>SNAMFTTVITPRVSETDGVGHINNTTVPVWFEAGRHEIFKLFTPDLSFKRW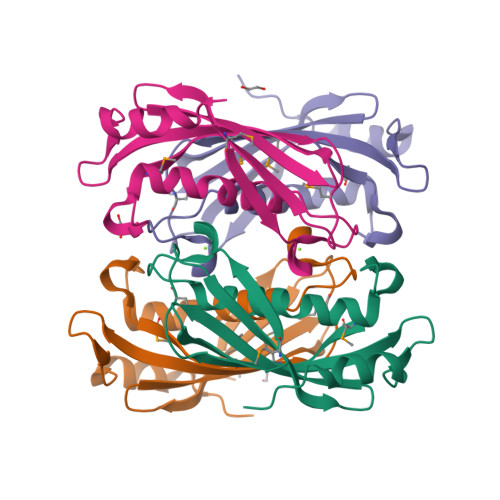RMVIIRMEVDYVNQMYYGQDVTVYTGIERIGNTSLTIYEEIHQNGVVCAKGRSVYVNFNFDTGRPEPIPDDIRVKLREHVWQPGE[4x]Mammals obtain nitrogen via the uptake of di- and tri-peptides in the gastrointestinal tract through the action of PepT1 and PepT2, which are members of the POT family of proton-coupled oligopeptide transporters. However, a key structural difference exists between bacterial and mammalian homologs with only the latter containing a large extracellular domain, the function of which is currently unknown. Here, we present the crystal structure of the extracellular domain from both PepT1 and PepT2 that reveal two immunoglobulin-like folds connected in tandem, providing structural insight into mammalian peptide transport. Functional and biophysical studies demonstrate that these domains interact with the intestinal protease trypsin, suggesting a role in clustering proteolytic activity to the site of peptide transport in eukaryotic cells.

Following extensive screening, crystals from Rattus norvegicus PepT2, residues 410–601, were also obtained. The phases were calculated from seleno-L-methionine incorporated protein using the SAD method in space group P3221. A higher-resolution structure in space group P41212 was obtained using the P3221 crystals as seeds with a single monomer in the asymmetric unit. The final structure refined to a resolution of 2.06 Å with final Rwork and Rfree of 19.9% and 24.0%, respectively. The crystallographic asymmetric unit of the PepT1ECD crystal contained two monomers that formed a head-to-tail dimer, related by a two-fold non-crystallographic symmetry axis, whereas the PepT2ECD construct was crystallized in a monomeric state. The crystal structures revealed that in the PepT1ECD there exist two conserved salt bridge interactions stabilizing the interface between lobe 1 and lobe 2, mediated by Asp574-Lys398 and Asp476-Arg490, whereas in PepT2ECD only one equivalent salt bridge interaction is present, between Asp505 and Arg538. Guinier analysis of the scattering data in PRIMUS (Petoukhov et al., 2007) shows that PepT2ECD has a larger radius of gyration (Rg) compared with PepT1ECD, 23.1 versus 18.4 Å, which suggests an increase in particle size. Consistent with this analysis, 3D envelopes of the ECD generated using DAMMIF show that PepT1ECD forms a compact shape ∼48 Å in length whereas PepT2ECD is more elongated, approximately 61 Å in length. The larger envelope of PepT2ECD indicates that the two immunoglobulin-like domains are structurally more dynamic than the PepT1ECD, which is consistent with the loss of the second salt bridge and also the location of Asp505 on the unstructured loop connecting lobes 1 and 2. We identified two highly conserved charged residues, Asp550 and Glu573 in PepT1ECD and Asp576 and Glu599 in PepT2ECD, located on one face of the ECD structure.

> MAASQEIFLQVLNLADGDVKVTVLGSRNNSLLVESVSSFQNTTHYSKLHLEAKSQDLHFHLKYNSLSVHNDHSVEEKNCYQLLIHQDGESISSMLVKDTGIKPANGMAAIRFINTLHKDLNISLDTDAPLSVGKDYGVSAYRTVLRGKYPAVHCETEDKVFSLDLGQLDFGTTYLFVITNITSQGLQAWKAEDI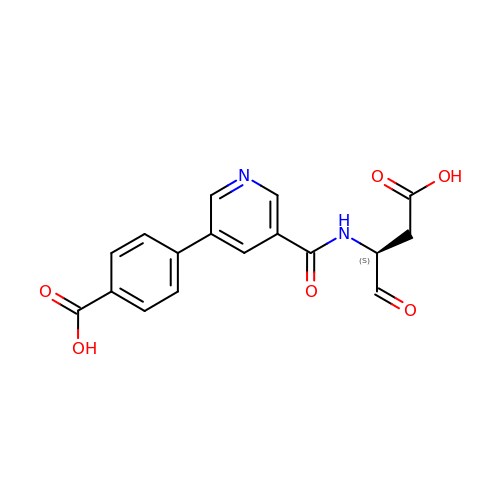4-[5-(2-CARBOXY-1-FORMYL-ETHYLCARBAMOYL)-PYRIDIN-3-YL]-BENZOIC ACID | C17 H14 N2 O6 | JNRAPROKLOUIRA-AWEZNQCLSA-N>[4x]MAEFRIAQDVVAREN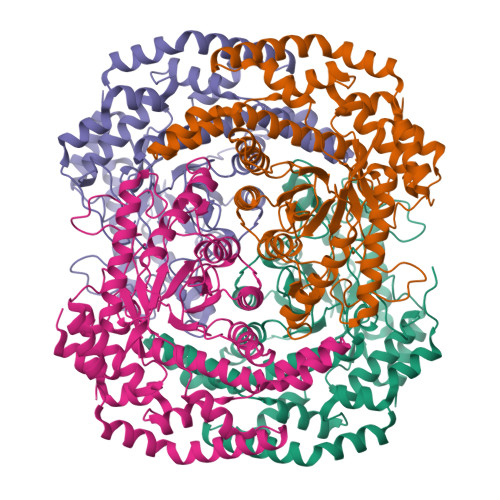DRRASALKEDYEALGANLARRGVDIEAVTAKVEKFFVAVPSWGVGTGGTRFARFPGTGEPRGIFDKLDDCAVIQQLTRATPNVSLHIPWDKADPKELKARGDALGLGFDAMNSNTFSDAPGQAHSYKYGSLSHTNAATRAQAVEHNLECIEIGKAIGSKALTVWIGDGSNFPGQSNFTRAFERYLSAMAEIYKGLPDDWKLFSEHKMYEPAFYSTVVQDWGTNYLIAQTLGPKAQCLVDLGHHAPNTNIEMIVARLIQFGKLGGFHFNDSKYGDDDLDAGAIEPYRLFLVFNELVDAEARGVKGFHPAHMIDQFHNVTDPIESLINSANEIRRAYAQALLVDRAALSGYQEDNDALMATETLKRAYRTDVEPILAEARRRTGGAVDPVATYRASGYRARVAAERPASVAGGGGIIGSHHHHHH The crystal structure of PA1994 from Pseudomonas aeruginosa, a member of the Pfam PF06475 family classified as a domain of unknown function (DUF1089), reveals a novel fold comprising a 15-stranded β-sheet wrapped around a single α-helix that assembles into a tight dimeric arrangement. The remote structural similarity to lipoprotein localization factors, in addition to the presence of an acidic pocket that is conserved in DUF1089 homologs, phospholipid-binding and sugar-binding proteins, indicate a role for PA1994 and the DUF1089 family in glycolipid metabolism. Genome-context analysis lends further support to the involvement of this family of proteins in glycolipid metabolism and indicates possible activation of DUF1089 homologs under conditions of bacterial cell-wall stress or host–pathogen interactions. The PA1994 gene of Pseudomonas aeruginosa, an opportunistic human pathogen, encodes a protein with a molecular weight of 21.6 kDa (residues 1–187) and a calculated isoelectric point of 4.9.

The final model includes 370 residues (residues 2–187 of chain A and residues 4–187 of chain B), nine ethylene glycol molecules, two MPD molecules and 367 water molecules in the asymmetric unit. The two outliers, Pro106 in chains A and B, are actually found in a cis conformation in both chains and have clear electron density. PA1994 can be viewed as consisting of two subdomains: the first half of the β-sheet (β1′, β3–β8) and helix H1 (residues 1–98) compose the first domain, which packs against the other subdomain consisting of the second half of the β-sheet (β9–β15) and helix H2 (residues 99–187). An analysis of PA1994 using the CastP server revealed a deep pocket (15 × 6 × 7 Å) enclosed mainly by helix H2 and strand β7, with additional contributions made by strands β10–β12 and the loop between strands β14 and β15. However, the binding pocket is hydrophobic in LolA, whereas the PA1994 pocket is acidic, suggesting a more hydrophilic ligand. The entrance to the pocket in PA1994 forms a long and narrow groove (20 × 7 Å) composed of strictly or highly conserved hydrophobic residues (Ile102, Pro106, Pro108, Phe165, Leu170 and Ile178) and also involves the dimerization interface (Trp13), suggesting a hydrophobic component of the ligand and the likely requirement of dimerization for binding. Analytical size-exclusion chromatography in combination with static light scattering indicates that PA1994 is a dimer in solution. The extensive dimerization interface observed in the structure, in addition to the SEC/SLS data, suggest that a dimer is likely to be the bio­logically relevant oligomeric state of PA1994. The swapped β-strands appear to participate in stabilizing the conserved cavity.

>GMSRDRLYTWAGLWRSPSSSWEALRLEDDQAESQLRAPDERSGLPYQLDYRLRWDADWHLREAVFHVESETGVRKLHLLADGRGHWQDGDGEALPAFDGCLDIDIWPSPFTNTFPIRRLGLADGQRAEIRALYIEAPALEPRSMRQAYTRLDASHYLYENLEGSAFKAVLLVDEQGLVIDYPGLFQRL[2x]>GYQNRTLRSITSPLVAHRLKPIRQKTKKAVVSILDSEEVCVELVKEYASQEYVKEVLQISSDGNTITIYYPNGGRGFPLADRPPSPTDNISRYSFDNLPEKYWRKYQYASRFVQLVRSKSPKITYFTRYAKCILMENSPGADFEVWFYDGVKIHKTEDFIQVIEKTGKSYTLKSESEVNSL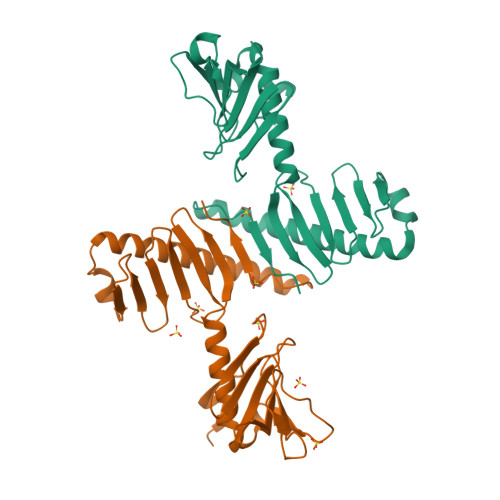KEEIKMYMDHANEGHRICLALESIISEEERKTRSAPFFPIIIGRKPG[2x]>YTVEPVQDGERSVTLRRAGGTPLVAAMYHLPAAGSPDFVGLDLAATILADTPSGRLYHALVPTKLASGVFGFTMDQLDPGLAMFGAQLQPGMDQDKALQTLTATLESLSSKPFSQEELERARSKWLTAWQQTYADPE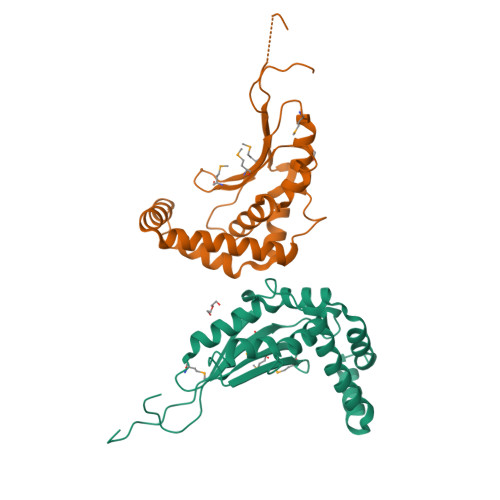KVGVALSEAIASGDWRLFFLQRDRVRDAKLDDVQRAAVAYLVRSNRTEGRYIPTEKPQRAPLAQRADLAAV[2x]> IVGGTASVRGEWPWQVTLHTTSPTQRHLCGGSIIGNQWILTAA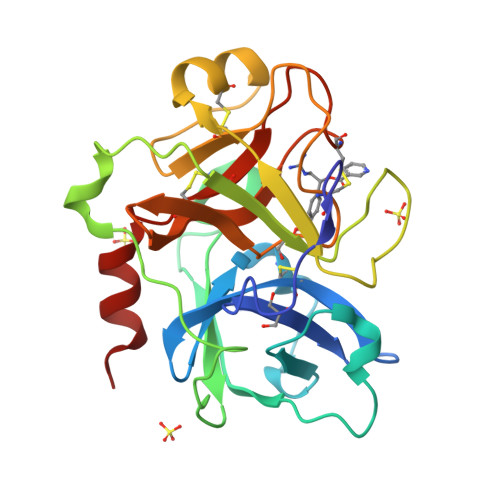HCFYGVESPKILRVYSGILNQAEIAEDTSFFGVQEIIIHDQYKMAESGYDIALLKLETTVNYADSQRPISLPSKGDRNVIYTDCWVTGWGYRKLRDKIQNTLQKAKIPLVTNEECQKRYRGHKITHKMICAGYREGGKDACKGDSGGPLSCKHNEVWHLVGITSWGEGCAQRERPGVYTNVVEYVDWILEKTQA2'-amino[1,1'-biphenyl]-2,3-diol 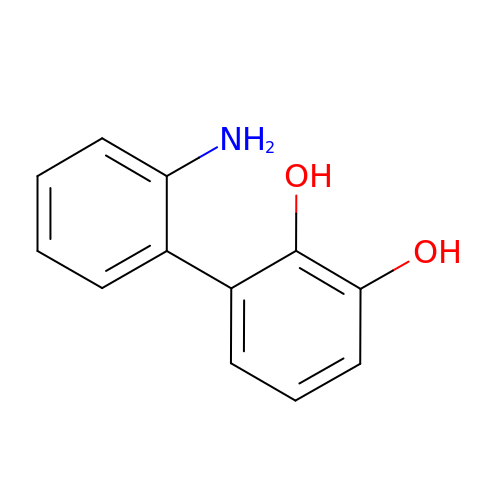| C12 H11 N O2 | WPDDFIBFWKUENN-UHFFFAOYSA-N> AVSFIGSTEN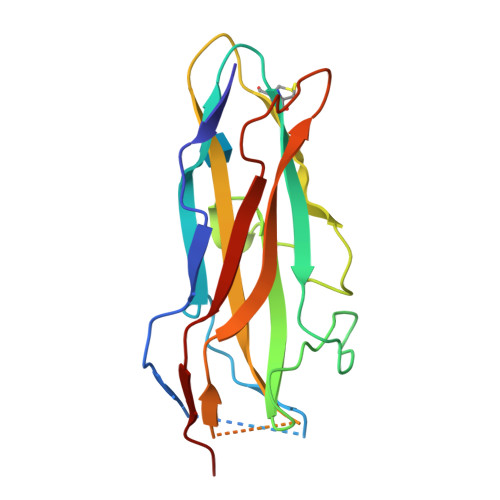DVGPSQGSYSRTHAMDNLPFVYDTGYNIGYQNANVWHISGGFCVGLDGKVDLPVVGSLDGQSIYGLTEEVGLLIWMGDTNYSRGTAMSGNSWENVFSGWCVGNYVSTQGLSVHVRPVILKRNSSAQYSVQKTSIGSIRMRPYNGSSAGSVQTTVNFSLNPFTLNDT> MLWCTGPRRIVFHNAPSVYPFTKPFHDTPYDQDRGRFDKTKNILRENKWPAWMDHGADGTGFGIGLNRTHPLSKLRGNLRRNPSEIPRVLNMMIQGVWHKSGNKLYFRGGKPPNPSTHPYLTGEPCPVYGWKVTDPGVIREFNLPQPEDKTRYKPYVALQERKIMGMQAPTKEHSAASTSAASTDSKPLMKRLF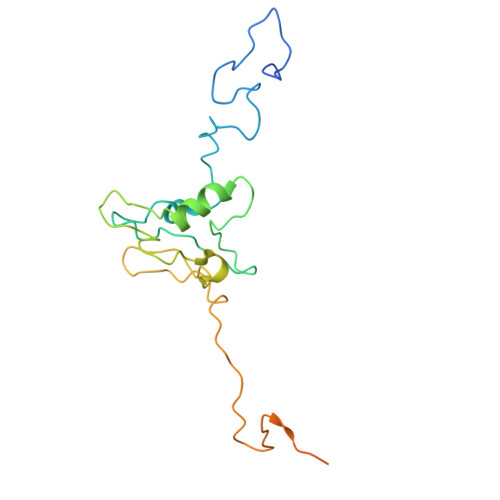FWK>MGSDSIDTPNYDVQKHINKLCGMLLITEDANHKFTGLIGMLYAMSRLGREDTIKILRDAGYHVKANGVDVTTHRQDINGKEMKFEVLTLASLTTEIQINIEIESRKSYKKMLKEMGEVAPEYRHDSPDCGMIILCIAALVITKLAAGDRSGLTAVIRRANNVLKNEMKRYKGLLPKDIANSFYEVFEKHPHFIDVFVHFGIAQSSTRGGSRVEGIFAGLFMNAYGLEHHH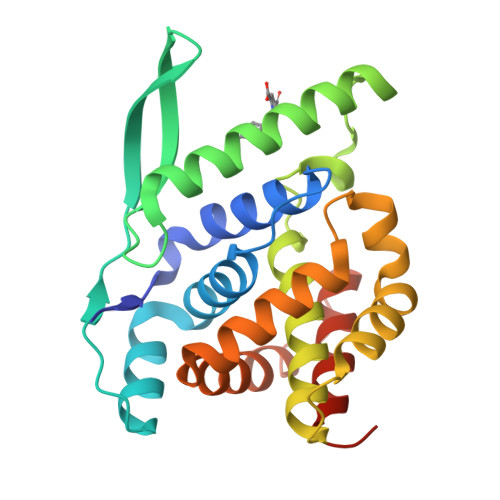HHH[2x]Thymidylate synthase (TS, EC 2.1.1.45) is a ubiquitous enzyme that catalyzes the reductive methylation of 2′-deoxyuridine-5′-monophosphate (dUMP) to 2′-deoxythymidyne-5′-monophosphate (dTMP) using N5,N10-methylenetetrahydrofolate (mTHF) as a cofactor. In cells, TS provides the only synthetic source of dTMP necessary for DNA biosynthesis. TS works as an obligate homodimer, having residues from both enzyme subunits that contribute to substrate binding in each catalytic site. TS subunits are characterized by two domains, known as large and small domains (LD and SD, respectively).

The structure of EfTS in complex with the substrate analogue FdUMP was determined at 2.88 Å resolution, consistently showing subunit asymmetry within each enzyme dimer. FdUMP populates the active sites of subunits B and D turned to a closed state, whereas chains A and C remain in the open conformation typical of ligand-free subunits. In subunits B and D, FdUMP binding is accompanied by the accommodation of 5-FTHF in the cofactor site (the same cofactor analogue also entrapped in the active site of the native enzyme). FdUMP occupies the substrate pocket, where it mimics the dUMP binding mode, forming similar interactions within the cavity. Nonetheless, the 5-fluoro-uracil moiety of FdUMP is positioned closer to the catalytic Cys197 (distance of ~2.7 Å between the inhibitor C6 and the cysteine thiol). On the contrary, in the complex with FdUMP, the thiol of Cys197 is reactive and can form a covalent adduct with the inhibitor that, indeed, is positioned closer to the catalytic residue. In this arrangement, the 5-fluorine on the FdUMP uracil moiety is proximal (~2.7 Å) to the Tyr145 hydroxyl, suggesting the formation of a halogen bond with it. Indeed, the pteridin moiety of 5-FTHF is accommodated just above the 5-fluoro-uracil of the substrate analogue, placing its 5-formyl substituent proximal to the FdUMP C5 (distance of ~3.2 Å). In EfTS, 5-FTHF, having a 5-formyl group that replaces the methyl of the cofactor, acts as an inhibitor, preventing the formation of the ternary covalent adduct. Therefore, our EfTS-FdUMP-5-FTHF ternary complex mimics the pre-reactive step of catalysis in which both substrate and cofactor are aligned in the cavity to allow the transfer of the pterin N-5 substituent.

>[4x]MEEAYLALGKKILEEGHFKEDRTGTGTYSLFGYQMRFDLAKGFPLLTTKRVPFGLIKSELLWFLKGDTNIRYLLERNNHIWDEWAFERYVKSADYQGPDMTDFGHRVLQDPAFAEQYKEEHQKFCDAILNDAEFAEKYGELGNIYGAQWRHWETKDGSFIDQLANVIEMIKTNPDSRRLIVSAWNPEDVPSMALPPCHTMFQFYVNEGKLSCQLYQRSADVFLGVPFNIASYALLTHLIAHETGLEVGEFVHTLGDAHLYQNHVEQMQEQLSREVRSFPTLVLNPDKASVFDFDMEDIKVEGYDPHPTIKAPIAV>MPACCSCSDVFQYETNKVTRIQSMNYGTIKWFFHVIIFSYVCFALVSDKLYQRKEPVISSVHTKVKGIAEVKEEIVENGVKKLVHSVFDTADYTFPLQGNSFFVMTNFLKTEGQEQRLCPEYPTRRTLCSSDRGCKKGWMDPQSKGIQTGRCVVYEGNQKTCEVSAWCPIEAVEEAPRPALLNSAENFTVLIKNNIDFPGHNYTTRNILPGLNITCTFHKTQNPQCPIFRLGDIFRETGDNFSDVAIQGGIMGIEIYWDCNLDRWFHHCRPKYSFRRLDDKTTNVSLYPGYNFRYAKYYKENNVEKRTLIKVFGIRFDILVFGTGGKFDIIQLVVYIGSTLSYFGLAAVFIDFLIDTYSSNCCRSHIYPWCKCCQPCVVNEYYYRKKCESIVEPKPTLKYVSFVDESHIRMVNQQLLGRSLQDVKGQEVPRPAMDFTDLSRLPLALHDTPPIPGQPEEIQLLRKEATPRSRDSPVWCQCGSCLPSQLPESHRCLEELCCRKKPGACITTSELFRKLVLSRHVLQFLLLYQEPLLALDVDSTNSRLRHCAYRCYATWRFGSQDMADFAILPSCCRWRIRKEFPKSEGQYSGFKSPY[3x]

The P2X7 receptor is an ATP-gated ion channel that activates inflammatory pathways involved in diseases such as cancer, atherosclerosis, and neurodegeneration. When present in high concentrations, such as in pathological inflammatory states, extracellular ATP acts as a danger signal to cells by binding to and activating the P2X7 receptor (P2X7R). This spatiotemporal signaling stimulates the innate immune system by triggering assembly of the NLRP3 inflammasome and subsequent cytokine release, as well as activation of various less understood signaling cascades, ultimately resulting in apoptosis. P2X7R antagonists bind to either classical or extended allosteric ligand-binding sites that exist within the extracellular domain at the interface of two protomers.

To gain molecular insight into the binding of ATP to hP2X7Rs, we determined the cryo-EM structure of the full-length wild-type hP2X7R in the ATP-bound open state at 3.0 Å resolution. The minimum pore radius of the hP2X7R in the ATP-bound open state is 2.5 Å, the same as the rP2X7R in the ATP-bound open state, and large enough to pass partially hydrated sodium ions such as those present in the closed pores of human, mouse, and rat P2X7Rs. Although there are structural similarities within the extracellular domains, the pore and cytoplasmic domains of the hP2X7R in the ATP-bound open state are rotated in comparison to the rP2X7R in the ATP-bound open state. Relative to the rP2X7R, TM1 of the hP2X7R is rotated up in-plane by ~7° and TM2 is rotated up in-plane by ~6° with the hinges at the extracellular ends of TM1 and TM2, respectively. The rotation of TM2 is further propagated into a global rotation of the cytoplasmic ballast by ~10° in the hP2X7R relative to the rP2X7R. This twist in the pore and cytoplasmic domain, much like the tightening of a spring, decreases the overall height of the hP2X7R by ~4 Å compared to the rP2X7R (distance between Cα carbons of residues 514 and 521), likely representing an inherent flexibility of the transmembrane and cytoplasmic domains in the ATP-bound open state conformation. In the ATP-bound open state of the hP2X7R, ATP is coordinated by the seven residues that are conserved in the orthosteric pocket of all P2XR subtypes: K64, K66, T189, K193, N292, R294, and K311. In addition, the hP2X7R-specific residues, L191, I214, and Y288, form hydrophobic interactions with the ribose group and the side chain of Q143 interacts with the 2′-hydroxy on the ribose group (3.3 Å). Of these subtype-specific residues, I214 and Y288 in hP2X7Rs are not conserved across P2X7R orthologs. No cryo-EM density for CHS was present in the structures of the mP2X7R and the rP2X7R in the apo closed state or the hP2X7R in the ATP-bound open state.>SMSNTISDRIVARSVIEAARFIQSWEDADPDSLTEDQVLAAAGFAARLHEGLQATVLQRLVDESNHEEYREFKAW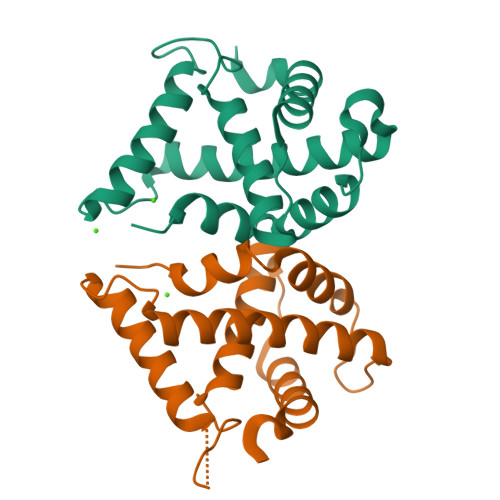EEALLNADGRVASSPFADWGWWYRIANVMLATASQNVGVTWGSRVHGRLMAIFQDKFKQRYEEQA[2x]> MKSRYTTEFHELEKIGSGEFGSVFKCVKRLDGCIYAIKRSKKPLAGSVDEQNALREVYAHAVLGQHSHVVRYFSAWAEDDHMLIQNEYCNGGSLADAISENYRIMSYFKEAELKDLLLQVGRGLRYIHSMSLVHMDIKPSNIFISRTSIPNAASEEGDEDDWASNKVMFKIGDLGHVTRISSPQVEEGDSRFLAN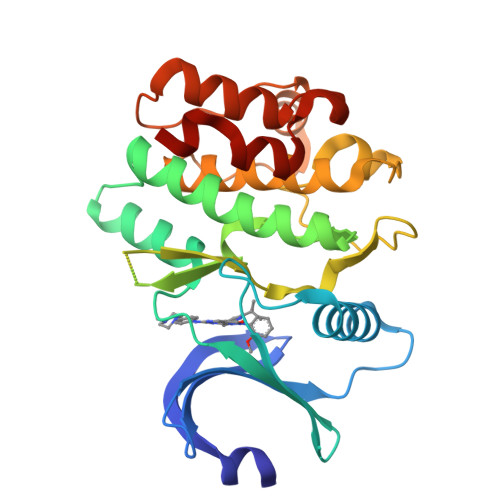EVLQENYTHLPKADIFALALTVVCAAGAEPLPRNGDQWHEIRQGRLPRIPQVLSQEFTELLKVMIHPDPERRPSAMALVKHSVLLSASRK3,5-dimethylpyrazin-2-ol 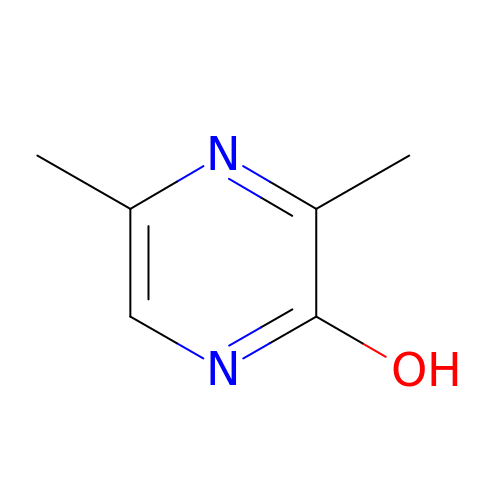| C6 H8 N2 O | AJYKJVCIKQEVCF-UHFFFAOYSA-N>[2x]GAGRHPPVVLVPGDLGNQLEAKLDKPTVVHYLCSKKTESYFTIWLNLELLLPVIIDCWIDNIRLVYNKTSRATQFPDGVDVRVPGFGKTFSLEFLDPSKSSVGSYFHTMVESLV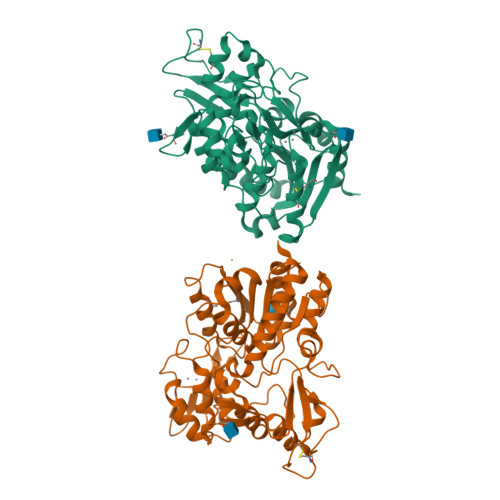GWGYTRGEDVRGAPYDWRRAPNENGPYFLALREMIEEMYQLYGGPVVLVAHSMGNMYTLYFLQRQPQAWKDKYIRAFVSLGAPWGGVAKTLRVLASGDNNRIPVIGPLKIREQQRSAVSTSWLLPYNYTWSPEKVFVQTPTINYTLRDYRKFFQDIGFEDGWLMRQDTEGLVEATMPPGVQLHCLYGTGVPTPDSFYYESFPDRDPKICFGDGDGTVNLKSALQCQAWQSRQEHQVLLQELPGSEHIEMLANATTLAYLKRVLLGP>[2x]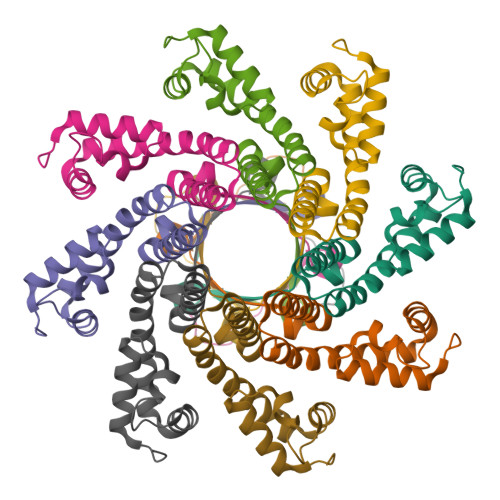GSHMATEPKAGRPSDYMPEVADDICSLLSSGESLLKVCKRPGMPDKSTVFRWLAKHEDFRDKYAKATEARADSIFEEIFEIADNAIPDAAEVAKARLRVDTRKWALARMNPRKYGDKVTNELVGKDGGAIQIETSPMSTLFGK>[4x]MHHHHHHGSSKLKKLSEDSLTKQPEEVFDVLEKLGEGSYGSVFKAIHKESGQVVAIKQVPVESDLQEIIKEISIMQQCDSPYVVKYYGSYFKNTDLWIVMEYCGAGSVSDIIRLRNKTLIEDEIATILKSTLKGLEYLHFMRKIHRNIKAGNILLNTEGHAKLADFGVAG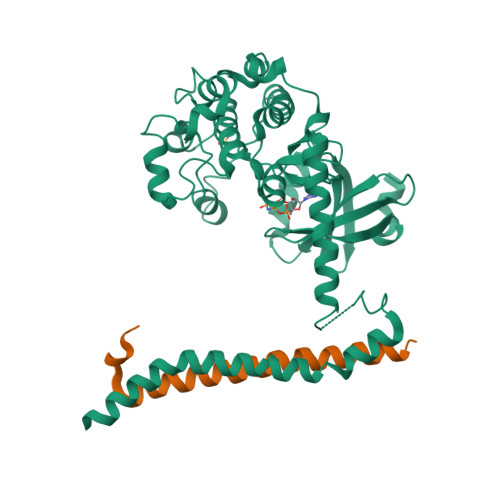QLTDTMAKRNTVIGTPFWMAPEVIQEIGYNCVADIWSLGITSIEMAEGKPPYADIHPMRAIFMIPTNPPPTFRKPELWSDDFTDFVKKCLVKNPEQRATATQLLQHPFIKNAKPVSILRDLITEAMEIKAKRHEEQQRELEEEENWKVPQDGDFDFLKNLSLEELQMRLKALDPMMEREIEELRQRYTAKRQPILDAMDAKKRRQQNF;>[4x]GEVEWDAFSIPELQNFLTILEKEEQDKIQQVQKKYDKFRQKLEEALRES>SAATQAVPTPNQQPEVLYNQIFINNEWHDAVSKKTFPTVNPSTGDVICHVAEGDKADVDRAVKAARAAFQLGSPWRRMDASERGRLLNRLADLIERDRTYLAALETLDNGKPYIISYLVDLDMVLKCLRYYAGWADKYHGKTIPIDGDYFSYTRHEPVGVCGQIIPWNFPLLMQAWKLGPALATGNVVVMKVAEQTPLTALYVANLIKEAGFPPGVVNVIPGFGPTAGAAIASHEDVDKVAFTGSTEVGHLIQVAAGKSNLKRVTLEIGGKSPNIIMSDADMDW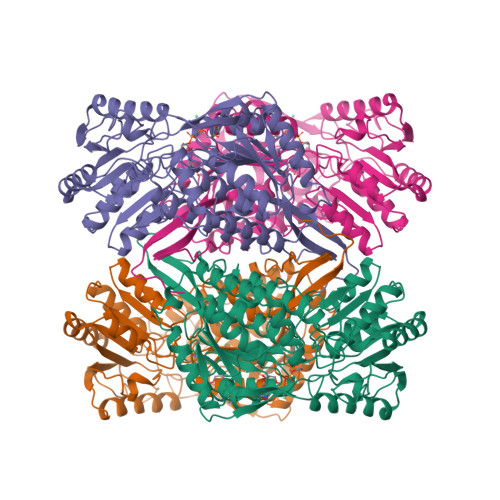AVEQAHFALFFNQGQCCCAGSRTFVQEDIYAEFVERSVARAKSRVVGNPFDSRTEQGPQVDETQFKKVLGYIKSGKEEGLKLLCGGGAAADRGYFIQPTVFGDLQDGMTIAKEEIFGPVMQILKFKSMEEVVGRANNSKYGLAAAVFTKDLDKANYLSQALQAGTVWVNCYDVFGAQSPFGGYKLSGSGRELGEYGLQAYTEVKTVTVRVPQKNS[4x]> GSIHVISRDQSTPIIEVEGPLLSDTHVTFKLTMPSPMPEYLNVHYICESASRLLFLSMHWARSIPAFQALGQDCNTSLVRACWNELFTLG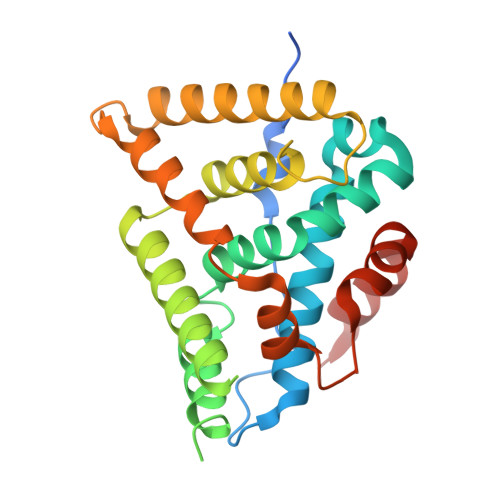LAQCAQVMSLSTILAAIVNHLQNSIQEDKLSGDRIKQVMEHIWKLQEFCNSMAKLDIDGYEYAYLKAIVLFSPDHPGLTSTSQIEKFQEKAQMELQDYVQKTYSEDTYRLARILVRLPALRLMSSNITEELFFTGLIGNVSIDSIIPYILKMETAEYNGQITGASL(1S,2S,3S,4R,5R)-2-amino-4-[benzyl(methyl)amino]-6,8-dioxabicyclo[3.2.1]octan-3-ol 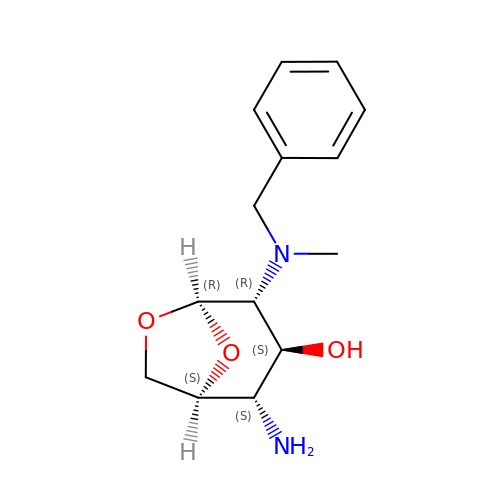| C14 H20 N2 O3 | YJSWHNBNNGQGQD-XGFWRYKXSA-N>[2x]UUGCG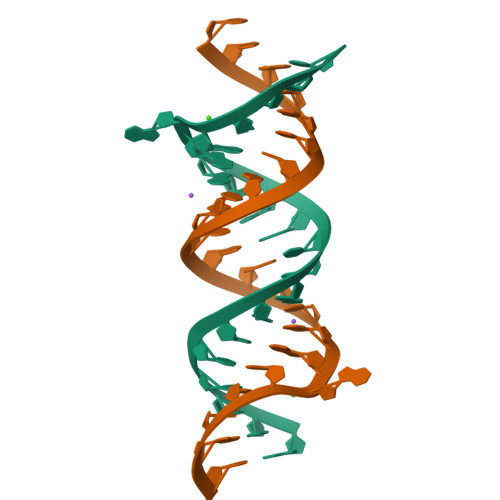UCUCGUCGACGAAGUCGC> MDALESLLDEVALEGLDGLCLPALWSRLETRVPPFPLPLEPCTQEFLWRALATHP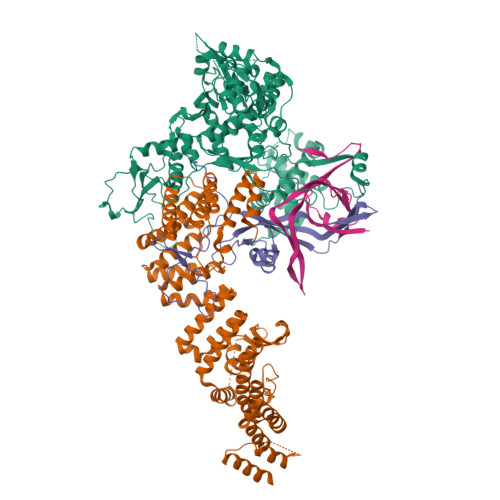GISFYEEPRERPDLQLQDRYEEIDLETGILESRRDPVALEDVYPIHMILENKDGIQGSCRYFKERKNITNDIRTKSLQPRCTMVEAFDRWGKKLIIVASQAMRYRALIGQEGDPDLKLPDFSYCILERLGRSRWQGELQRDLHTTAFKVDAGKLHYHRKILNKNGLITMQSHVIRLPTGAQQHSILLLLNRFHVDRRSKYDILMEKLSVMLSTRTNHIETLGKLREELGLCERTFKRLYQYMLNAGLAKVVSLRLQEIHPECGPCKTKKGTDVMVRCLKLLKEFKRNDHDDDEDEEVISKTVPPVDIVFERDMLTQTYDLIERRGTKGISQAEIRVAMNVGKLEARMLCRLLQRFKVVKGFMEDEGRQRTTKYISCVFAEESDLSRQYQREKARSELLTTVSLASMQEESLLPEGEDTFLSESDSEEERSSSKRRGRGSQKDTRASANLRPKTQPHHSTPTKGGWKVVNLHPLKKQPPSFPGAAEERACQSLASRDSLLDTSSVSEPNVSFVSHCADSNSGDIAVIEEVRMENPKESSSSLKTGRHSSGQDKPHETYRLLKRRNLIIEAVTNLRLIESLFTIQKMIMDQEKQEGVSTKCCKKSIVRLVRNLSEEGLLRLYRTTVIQDGIKKKVDLVVHPSMDQNDPLVRSAIEQVRFRISNSSTANRVKTSQPPVPQGEAEEDSQGKEGPSGSGDSQLSASSRSESGRMKKSDNKMGITPLRNYHPIVVPGLGRSLGFLPKMPRLRVVHMFLWYLIYGHPASNTVEKPSFISERRTIKQESGRAGVRPSSSGSAWEACSEAPSKGSQDGVTWEAEVELATETVYVDDASWMRYIPPIPVHRDFGFGWALVSDILLCLPLSIFIQIVQVSYKVDNLEEFLNDPLKKHTLIRFLPRPIRQQLLYKRRYIFSVVENLQRLCYMGLLQFGPTEKFQDKDQVFIFLKKNAVIVDTTICDPHYNLARSSRPFERRLYVLNSMQDVENYWFDLQCVCLNTPLGVVRCPRVRKNSSTDQGSDEEGSLQKEQESAMDKHNLERKCAMLEYTTGSREVVDEGLIPGDGLGAAGLDSSFYGHLKRNWIWTSYIINQAKKENTAAENGLTVRLQTFLSKRPMPLSARGNSRLNIWGEARVGSELCAGWEEQFEVDREPSLDRNRRVRGGKSQKRKRLKKDPGKKIKRKKKGEFPGEKSKRLRYHDEADQSALQRMTRLRVTWSMQEDGLLVLCRIASNVLNTKVKGPFVTWQVVRDILHATFEESLDKTSHSVGRRARYIVKNPQAYLNYKVCLAEVYQDKALVGDFMNRRGDYDDPKVCANEFKEFVEKLKEKFSSALRNSNLEIPDTLQELFARYRVLAIGDEKDQTRKEDELNSVDDIHFLVLQNLIQSTLALSDSQMKSYQSFQTFRLYREYKDHVLVKAFMECQKRSLVNRRRVNHTLGPKKNRALPFVPMSYQLSQTYYRIFTWRFPSTICTESFQFLDRMRAAGKLDQPDRFSFKDQDNNEPTNDMVAFSLDGPGGNCVAVLTLFSLGLISVDVRIPEQIIVVDSSMVENEVIKSLGKDGSLEDDEDEEDDLDEGVGGKRRSMEVKPAQASHTNYLLMRGYYSPGIVSTRNLNPNDSIVVNSCQMKFQLRCTPVPARLRPAAAPLEELTMGTSCLPDTFTKLINPQENTCSLEEFVLQLELSGYSPEDLTAALEILEAIIATGCFGIDKEELRRRFSALEKAGGGRTRTFADCIQALLEQHQVLEVGGNTARLVAMGSAWPWLLHSVRLKDREDADIQREDPQARPLEGSSSEDSPPEGQAPPSHSPRGTKRRASWASENGETDAEGTQMTPAKRPALQDSNLAPSLGPGAEDGAEAQAPSPPPALEDTAAAGAAQEDQEGVGEFSSPGQEQLSGQAQPPEGSEDPRGFTESFGAANISQAARERDCESVCFIGRPWRVVDGHLNLPVCKGMMEAMLYHIMTRPGIPESSLLRHYQGVLQPVAVLELLQGLESLGCIRKRWLRKPRPVSLFSTPVVEEVEVPSSLDESPMAFYEPTLDCTLRLGRVFPHEVNWNKWIHLGGGSGGGSGGSLEVLFQGPGSGSDYKDDDDKGDYKDDDDKGDYKDDDDK;> MSGFSPELIDYLEGKISFEEFERRREERKTREKKSLQEKGKLSAEENPDDSEVPSSSGINSTKSQDKDVNEGETSDGVRKSVHKVFASMLGENEDDEEEEEEEEEEEEEEETPEQPTAGDVFVLEMVLNRETKKMMKEKRPRSKLPRALRGLMGEANIRFARGEREEAILMCMEIIRQAPLAYEPFSTLAMIYEDQGDMEKSLQFELIAAHLNPSDTEEWVRLAEMSLEQDNIKQAIFCYTKALKYEPTNVRYLWERSSLYEQMGDHKMAMDGYRRILNLLSPSDGERFMQLARDMAKSYYEANDVTSAINIIDEAFSKHQGLVSMEDVNIAAELYISNKQYDKALEIITDFSGIVLEKKTSEEGTSEENKAPENVTCTIPDGVPIDITVKLMVCLVHLNILEPLNPLLTTLVEQNPEDMGDLYLDVAEAFLDVGEYNSALPLLSALVCSERYNLAVVWLRHAECLKALGYMERAAESYGKVVDLAPLHLDARISLSTLQQQLGQPEKALEALEPMYDPDTLAQDANAAQQELKLLLHRSTLLFSQGKMYGYVDTLLTMLAMLLKVAMNRAQVCLISSSKSGERHLYLIKVSRDKISDSNDQESANCDAKAIFAVLTSVLTKDDWWNLLLKAIYSLCDLSRFQEAELLVDSSLEYYSFYDDRQKRKELEYFGLSAAILDKNFRKAYNYIRIMVMENVNKPQLWNIFNQVTMHSQDVRHHRFCLRLMLKNPENHALCVLNGHNAFVSGSFKHALGQYVQAFRTHPDEPLYSFCIGLTFIHMASQKYVLRRHALIVQGFSFLNRYLSLRGPCQESFYNLGRGLHQLGLIHLAIHYYQKALELPPLVVEGIELDQLDLRRDIAYNLSLIYQSSGNTGMAQTLLYTYCSI;> MHHHHHHENLYFQGMAAEAADLGLGAAVPVELRRERRMVCVEYPGVVRDVAKMLPTLGGEEGVSRIYADPTKRLELYFRPKDPYCHPVCANRFSTSSLLLRIRKRTRRQKGVLGTEAHSEVTFDMEILGIISTIYKFQGMSDFQYLAVHTEAGGKHTSMYDKVLMLRPEKEAFFHQELPLYIPPPIFSRLDAPVDYFYRPETQHREGYNNPPISGENLIGLSRARRPHNAIFVNFEDEEVPKQPLEAAAQTWRRVCTNPVDRKVEEELRKLFDIRPIWSRNAVKANISVHPDKLKVLLPFIAYYMITGPWRSLWIRFGYDPRKNPDAKIYQVLDFRIRCGMKHGYAPSDLPVKAKRSTYNYSLPITVKKTSSQLVTMHDLKQGLGPSGTSGARKPASSKYKLKDSVYIFREGALPPYRQMFYQLCDLNVEELQKIIHRNDGAENSCTERDGWCLPKTSDELRDTMSLMIRQTIRSKRPALFSSSAKADGGKEQLTYESGEDEEDEEEEEEEEEDFKPSDGSENEMETEILDYV;> MAAAADERSPEDGEDEEEEEQLVLVELSGIIDSDFLSKCENKCKVLGIDTERPILQVDSCVFAGEYEDTLGTCVIFEENVEHADTEGNNKTVLKYKCHTMKKLSMTRTLLTEKKEGEENIGGVEWLQIKDNDFSYRPNMICNFLHENEDEEVVASAPDKSLELEEEEIQMNDSSNLSCEQEKPMHLEIEDSGPLIDIPSETEGSVFMETQMLP3-(2-{5-TERT-BUTYL-3-[(4-METHYL-FURAZAN-3-YLMETHYL)-AMINO]-2-OXO-2H-PYRAZIN-1-YL}-BUTYRYLAMINO)-5-(HEXYL-METHYL-AMINO)-4-OXO-PENTANOIC ACID ANION | C28 H44 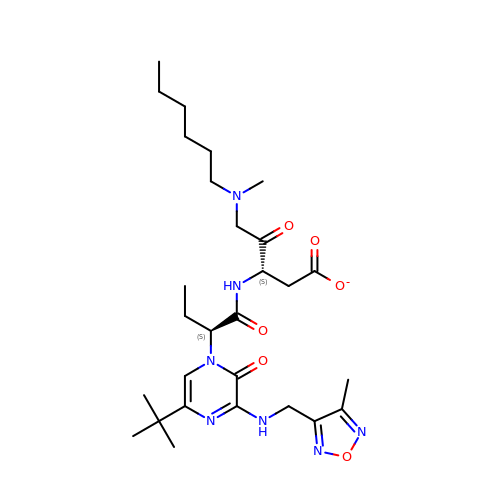N7 O6 | XIMITGPWYYFUQF-FPOVZHCZSA-M>[4x]GPLGQGQPRELAGCGSRADGGFRPSRVVVVAKTTRYEFEQQRYRYAE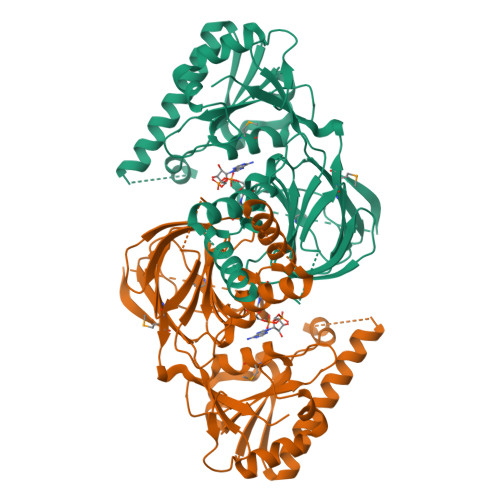LSEEDLKQLLALKGSSYSGLLERHHIHTKNVEHIIDSLRNEGIEVRLVKRREYDEETVRWADAVIAAGGDGTMLLAASKVLDRLKPVIGVNTDPERSEGHLCLPVRYTHSFPEALQKFYRGEFRWLWRQRIRLYLEGTGINPVPVDLHEQQLSLNQHNRALNIERAHDERSEASGPQLLPVRALNEVFIGESLSSRASYYEISVDDGPWEKQKSSGLNLCTGTGSKAWSFNINRVATQAVEDVLNIAKRQGNLSLPLNRELVEKVTNEYNESLLYSPEEPKILFSIREPIANRVFSSSRQRCFSSKVCVRSRCWDACMVVDGGTSFEFNDGAIASMMINKEDELRTVLLEQ> TKPYSSPPTNLRSLRDRLTQVAERQGVVFGRLQRHVAMIVVAQFAATLTDDTGAPLLLVKGGSSLELRRGIPDSRTSKDFDTVARRDIELIHEQLADAGETGWEGFTAIFTAPEEIDVPGMPVKPRRFTAKLSYRGRAFATVPIEVSSVEAGNADQFDTLTSDALGLVGVPAAVAVPCMTIPWQIAQKLHAVTAVLEEPKVNDRAHDLVDLQLLEGLLLDADLMPTRSACIAIFEARAQHPW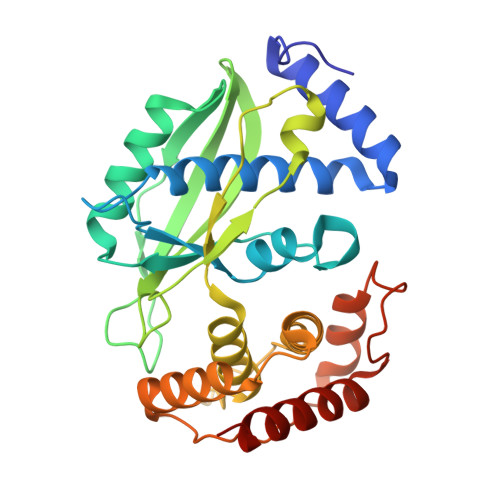PPRVATLPHWPLIYAGALEGLDHLELARTVDAAAQAVQRFVARIDRATKR> SGVSSPAPCPAPCACDLDGGADCSGKGLVTVPDGLSVFTHSLDLSMNNITKLPEGAFKGFPYLEELRLAGNDLSIIHPMALSGLKELKVLTLQNNQLKTVPSESLKGLVSLQSLRLDANH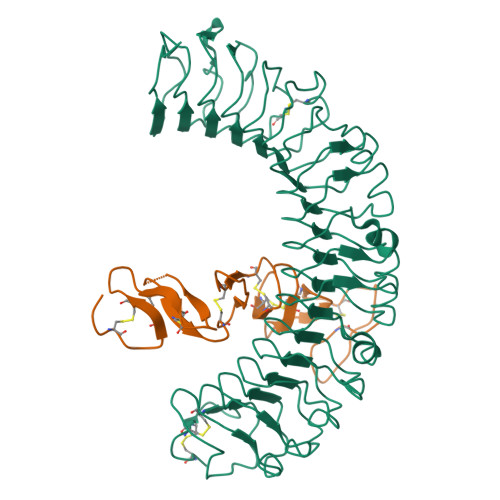IVTVPEDSFEGLVQLRHLWLDDNSLTEVPIRPLSNLPSLQALTLALNKISHIPDYAFSNLSSLVVLHLHNNKIRTLGPHSFHGLDNLEALDLNYNNLIDFPDSIRSLPNLKELGFHSNSITIIPDGAFVKNPLLRTIHLYDNPLSFVGNSAFQNLSDLHFLIIRGASNVQWFPNLTGTNNLESLTLTGTKIRSIPIKFCQEQKMLRTLDLSYNEISALVGFEGCSSLEEVYLQNNQIQEVQNETFQGLAALRMLDLSRNRIHTIHKEAFVTLKALTNLDLSFNDLTAFPTAGLHGLNQLKLTGNPNFKETLT;> SAEGSQACAKGCELCSEVNGCLKCSPKLFILLERNDIRQVGVCLPSCPPGYFDARNPDMNKCIKCKIEHCEACFSHNFCTKCKEGLYLHKGRCYPACPEGSSAANGTMECSS>[4x]MAHHHHHHMAATKLGINGFGRIGRLVFRAAFGRKDIEVVAINDPFMDLNHLCYLLKYDSVHGQFPCEVTHADGFLLIGEKKVSVFAEKDPSQIPWGKCQVDVVCESTGVFLTKELASSHLKGGAKKVIMSAPPKDDTPIYVMGINHHQYDTKQLIVSNASCTTNCLAPLAKVINDRFGIVEGLMTTVHASTANQLVVDGPSKGGKDWRAGRCALSNIIPASTGAAKAVGKVLPELNGKLTGVAFRV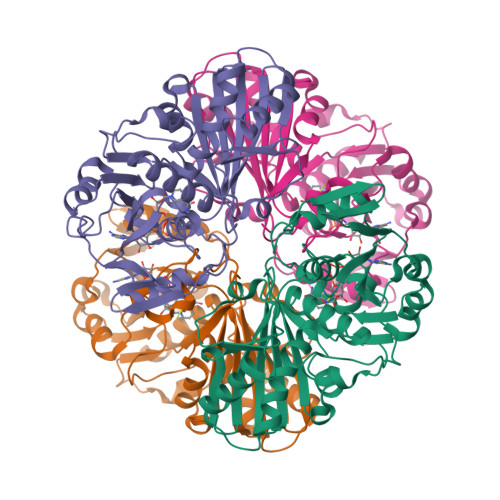PIGTVSVVDLVCRLQKPAKYEEVALEIKKAAEGPLKGILGYTEDEVVSQDFVHDNRSSIFDMKAGLALNDNFFKLVSWYDNEWGYSNRVLDLAVHITTS>EELPQIEIVQEGDNTTFAKPGDTVTIHYDGKLTNGKEFDSSRKRGKPFTCTVGVGQVIKGWDISLTNNYG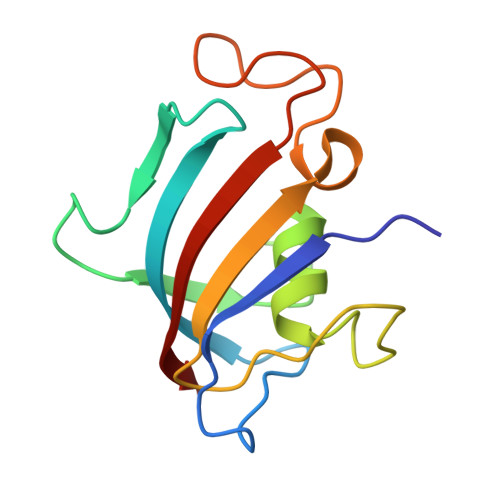KGGANLPKISKGTKAILTIPPNLAYGPRGIPGIIGPNETLVFEVELLGVN[2x]(3~{R})-3-(4-aminophenyl)-3-ethyl-piperidine-2,6-dione 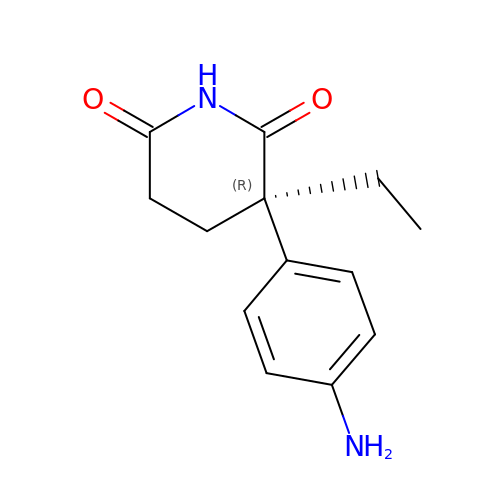| C13 H16 N2 O2 | ROBVIMPUHSLWNV-CYBMUJFWSA-N>[3x]GPLGSKQVFKNRKYPITDFEKYLQDITKVRGPMSIDTFIKEVLTNPKYGYYMNKDVFGKGGDFITAPEVSQLFGEMIGIWCVA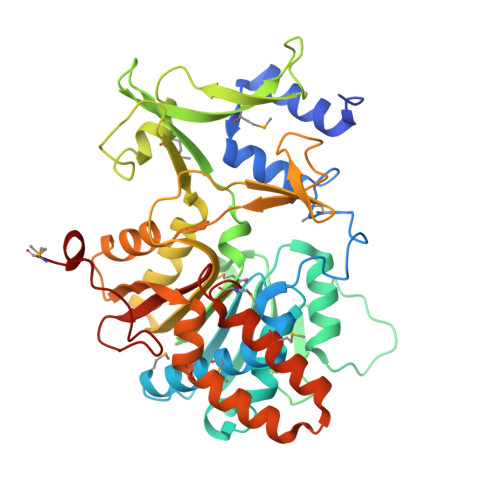TWEAMGKPKKLQIVEMGPGRGTLMKDILRSTKVFKEFYDSISVHLVEASPANKKTQKQNLLYFKDKAINFDHKTIGETPNGIKVTWVGKLEEVPTDIPTLFLAQEFFDALPIHVFRFSREKNDWCEVLVDEDITEHGEYYLRFVQSKGPTLMTTAVKHLLPEFGLDGYQVELGLAGLAISQQIANRIDKSGGAALIIDYGYDKIVKSSLQAIRDHEFVDILDKPGTADLSVWVDFQTIRKTVKLLKNKSTAIGPVDQGIFLKEMGIEHRLAQIGRKLDSNEKFEELVMGYKKLVDPKEMGTNYKVITICDKNITPIGFSTSKTYDDEDLMI>QSAKYHRLNLQNPAAAPFLESYKKAITVMLQLPPSDARNWYRNAFIHTLDCPHGNWWFVVWHRGYTGWFERTVRELSGDPNFAFPYWDWTALPQVPDSFFNGVLDPNNPAFIASYNEFYSQLSNPMSALWNSFSTAQLQQMRNRGFQSVNDVWQAVRDSPMFFPRGRARTLTRQNPGFDATTRRAVSIGTIRNALAPTDFITFGSGKTANHSESATQGILESQPHNNVHNNIGGFMQDLLSPTDPVFFAHHSNIDRLWDVWTRKQQRLGLPTLPTGANLPLWANEPFLFFIGPDGKPVAKNKAGDYATIGDFDYNYEPGSGEAV[2x]

Tyrosinases (EC.1.14.18.1) are bifunctional metalloenzymes catalyzing two sequential enzymatic reactions: hydroxylation of monophenols to o-diphenols (monophenolase activity) and oxidation of o-diphenols to the corresponding o-quinones (diphenolase or catecholase activity). The tyrosinase from the bacterium Verrucomicrobium spinosum (vsTyr) is produced as a pre-pro-enzyme in which a C-terminal extension serves as an inactivation domain. It does not require a caddie protein for copper ion incorporation, which makes it similar to eukaryotic tyrosinases. To gain an understanding of the catalytic machinery and regulation of vsTyr activity, we determined the structure of the catalytically active “core domain” of vsTyr by X-ray crystallography.

Crystals of the vsTyr core domain belong to the space group C2 containing two monomers per asymmetric unit. Despite reconstitution with CuSO4 after its purification, the initial crystal structure, determined by molecular replacement at 1.43 Å resolution, revealed that the copper sites were only partially occupied. A second dataset was therefore collected from a vsTyr crystal soaked with CuSO4 for 15 min (1.64 Å), resulting in considerably improved metal site occupancy. The vsTyr structure, determined from a crystal presoaked with CuSO4 for 15 min, revealed significantly increased metal site occupancies of 70–85% for site A and >90% for site B, respectively. For vsTyr, the distances of 3.7 Å and 4.0 Å observed in the structures determined from unsoaked and CuSO4-presoaked crystals, respectively, fall within the 3.2–4.0 Å range that is characteristic for the met form. Crystal soaking led to the appearance of anomalous density peaks on the protein surface, but outside the active site, that could be interpreted as additional Cu2+-binding sites. In the vsTyr crystals, this last site is located directly adjacent to the same site found in a neighboring symmetry mate. These additional binding sites are most likely not of any physiological relevance, since their affinities for Cu2+ are expected to be low, and none of them has to date been observed in homologous enzymes. Interestingly, the increased metal site occupancy is the only noticeable difference between the two vsTyr core domain structures reported here. Their superposition results in a very low RMSD of 0.4 Å and identical crystal packing, hinting at the remarkable structural stability of the vsTyr core domain. The final models contain all amino acids of the crystallized construct, except for the C-terminal two (unsoaked) and three amino acids (soaked) in chains B, respectively.>MERYESLFAQLKERKEGAFVPFVTLGDPGIEQSLKIIDTLIEAGADALELGIPFSDPLADGPTIQNATLRAFAAGVTPAQCFEMLALIRQKHPTIPIGLLMYANLVFNKGIDEFYAQCEKVGVDSVLVADVPVEESAPFRQAALRHNVAPIFICPPNADDDLLRQIASYGRGYTYLLSRAGVTGAENRAALPLNHLVAKLKEYNAAPPLQGFGISAPDQVKAAID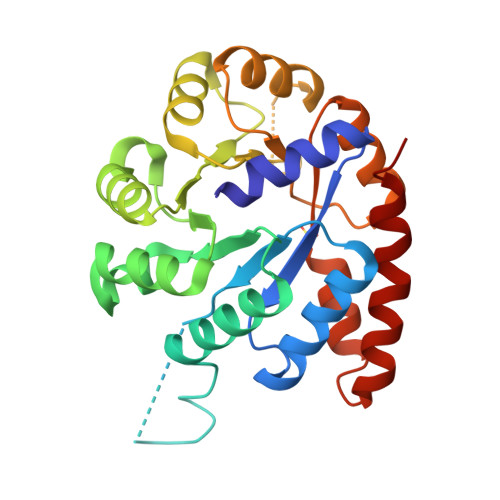AGAAGAISGSAIVKIIEQHINEPEKMLAALKVFVQPMKAATRS[2x]>MGSSHHHHHHSQDPSQFIRRDIAQTVNGSLTLTQQTNLSAPLVSSSTGEFGGSLAANRTFTIRNTGAPTSIVFEKGPASGANPAQSMSIRVWGNQFGGGSDTTRSTVFEVGDDTSHHFYSQRNKDGNIAFNINGTVMPININASGLMNVNGTATFGRSVTANGEFISKSANAFRAINGDYGFFIRNDASNTYFLLTAAGDQTGGFNGLRPLLINNQSGQITIGEGLIIAKGVTINSGGLTVNSRIRSQGTKTSDLYTRAPTSDTVGFWSIDINDSATYNQFPGYFKMVEKTNEVTGLPYLERGEEVKSPGTLTQFGNTLDSLYQDWITYPTTPEARTTRWTRTWQKTKNSWSSFVQVF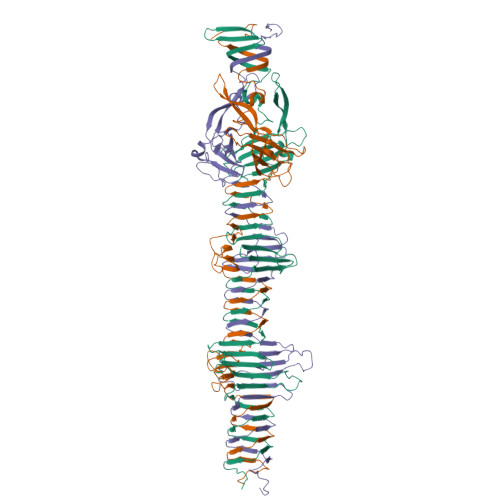DGGNPPQPSDIGALPSDNATMGNLTIRDFLRIGNVRIVPDPVNKTVKFEWVE[12x]>MTHVEVVATIAPQLYIEETLIQKINHRIDAIDVLELRIDQIENVTVNQVAEMITKLKVMQDSFKLLVTYRTKLQGGYGQFTNDLYLNLISDLANINGIDMIDIEWQADIDIEKHQRIITHLQQYNKEVVISHHNFESTPPLDELQFIFFKMQKFNPEYVKLAVMPHNKNDVLNLLQAMSTFSDTMDCKVVGISMSKLGLISRTAQGVFGG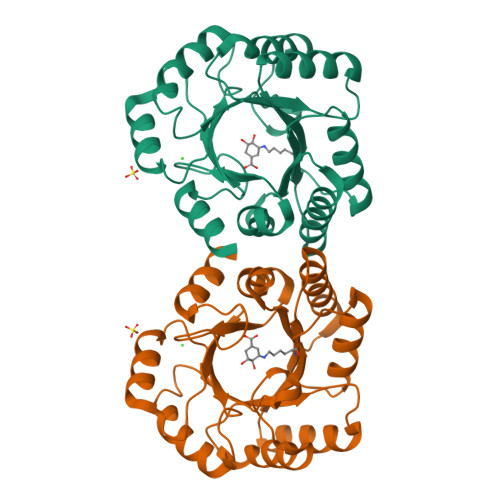ALTYGCIGEPQAPGQIDVTDLKAQVTLY[2x]>GRSRLLEDFRNNRYPNLQLREIAGHIMEFSQDQHGSRFIQLKLERATPAERQLVFNEILQAAYQLMVDVFGNYVIQKFFEFGSLEQKLALAERIRGHVLSLALQMYGCRVIQKALEFIPSDQQNEMVRELDGHVLKCVKDQNGNHVVQKCIECVQPQSLQFIIDAFKGQVFALSTHPYGCRVIQRILEHCLPDQTLPILEELHQHTEQLVQDQYGNYVIQHVLEHGRPEDKSKIVAEIRGNVLVLSQHKFASNVVEKCVTHASRTERAVLIDEVCTMND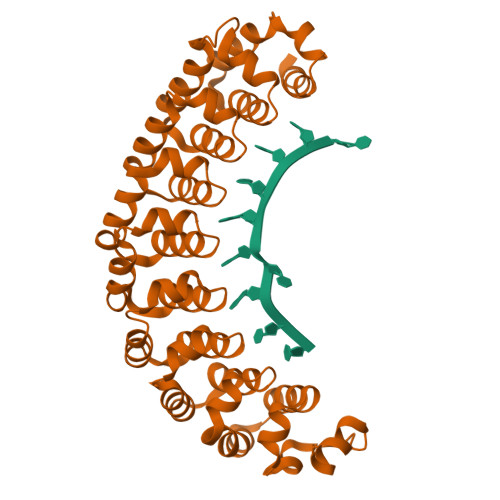GPHSALYTMMKDQYANYVVQKMIDVAEPGQRKIVMHKIRPHIATLRKYTYGKHILAKLEKYYMK[2x]>[2x]GGEVPIGDPKELNGMEIAAVYLQPIEMEPRGIDLAASLADIHLEADIHALKNNPNGFPEGFWMPYLTIAYELKNTDTGAIKR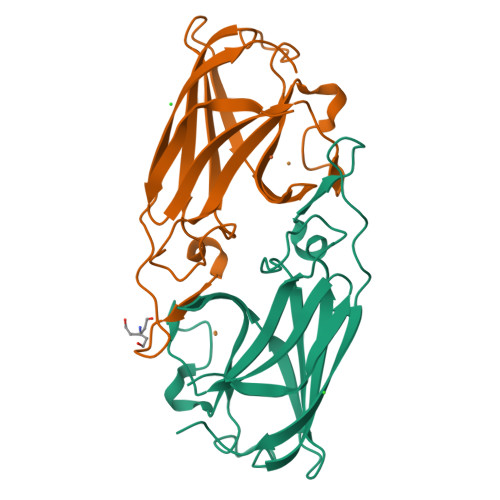GTLMPMVADDGPHYGANIAMEKDKKGGFGVGNYELTFYISNPEKQGFGRHVDEETGVGKWFEPFKVDYKFKYTGTPK>[2x]MFHSSAMVNSHRKPMFNIHRGFYCLTAILPQICICSQFSVPSSYHFTEDPGAFPVATNGERFPWQELRLPSVVIPLHYDLFVHPNLTSLDFVASEKIEVLVSNATQFIILHSKDLEITNATLQSEEDSRYMKPGKELKVLSYPAHEQIALLVPEKLTPHLKYYVAMDFQAKLGDGFEGFYKSTYRTLGGETRILAVTDFEPTQARMAFPCFDEPLFKANFSIKIRRESRHIALSNMPKVKTIELEGGLLEDHFETTVKMSTYLVAYIVCDFHSLSGFTSSGVKVSI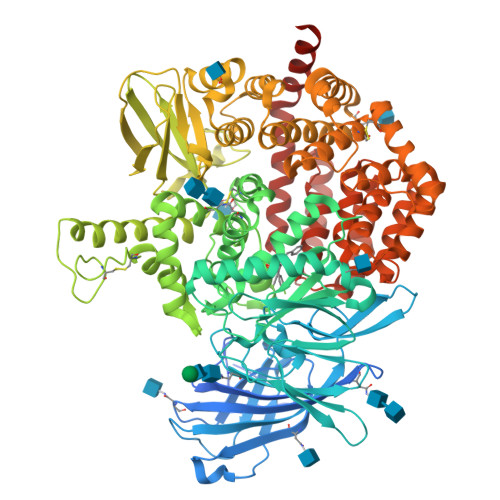YASPDKRNQTHYALQASLKLLDFYEKYFDIYYPLSKLDLIAIPDFAPGAMENWGLITYRETSLLFDPKTSSASDKLWVTRVIAHELAHQWFGNLVTMEWWNDIWLNEGFAKYMELIAVNATYPELQFDDYFLNVCFEVITKDSLNSSRPISKPAETPTQIQEMFDEVSYNKGACILNMLKDFLGEEKFQKGIIQYLKKFSYRNAKNDDLWSSLSNSCLESDFTSGGVCHSDPKMTSNMLAFLGENAEVKEMMTTWTLQKGIPLLVVKQDGCSLRLQQERFLQGVFQEDPEWRALQERYLWHIPLTYSTSSSNVIHRHILKSKTDTLDLPEKTSWVKFNVDSNGYYIVHYEGHGWDQLITQLNQNHTLLRPKDRVGLIHDVFQLVGAGRLTLDKALDMTYYLQHETSSPALLEGLSYLESFYHMMDRRNISDISENLKRYLLQYFKPVIDRQSWSDKGSVWDRMLRSALLKLACDLNHAPCIQKAAELFSQWMESSGKLNIPTDVLKIVYSVGAQTTAGWNYLLEQYELSMSSAEQNKILYALSTSKHQEKLLKLIELGMEGKVIKTQNLAALLHAIARRPKGQQLAWDFVRENWTHLLKKFDLGSYDIRMIISGTTAHFSSKDKLQEVKLFFESLEAQGSHLDIFQTVLETITKNIKWLEKNLPTLRTWLMVNTRHHHHHH METHANOL | C H4 O | 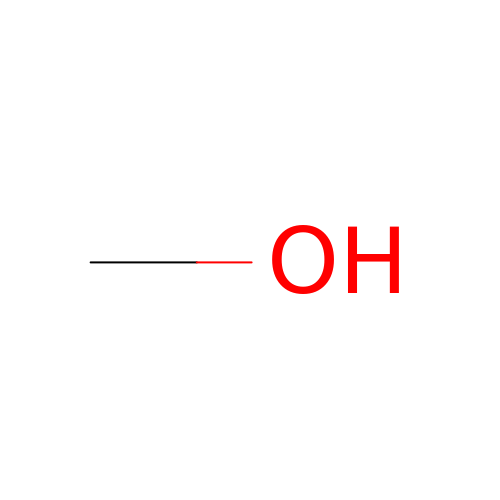OKKJLVBELUTLKV-UHFFFAOYSA-N1-ethanoyl-9~{H}-pyrido[3,4-b]indole-3-carboxylic 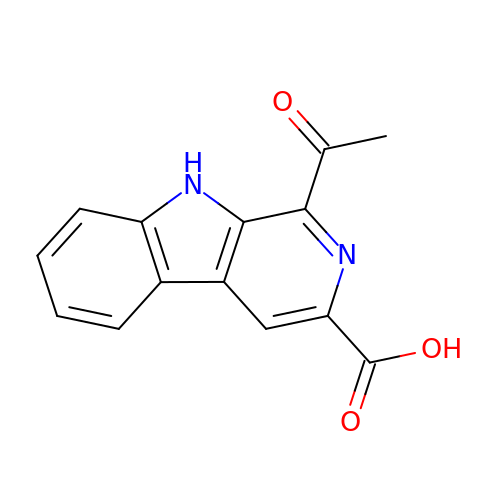acid | C14 H10 N2 O3 | RMLMLEMGHAUXDM-UHFFFAOYSA-N>[2x]AAAAALSTLSSTESLTISSNRTLVSPGNIFELGFFRTNSRWYLGMWYKKLSGRTYVWVANRDNPLSNSIGTLKISNMNLVLLDHSNKSVWSTNLTRENVRSPVVAELLANGNFVVRDPSGFLWQSFDYPTDTLLPEMKLGYDLKTGLNRFLVSW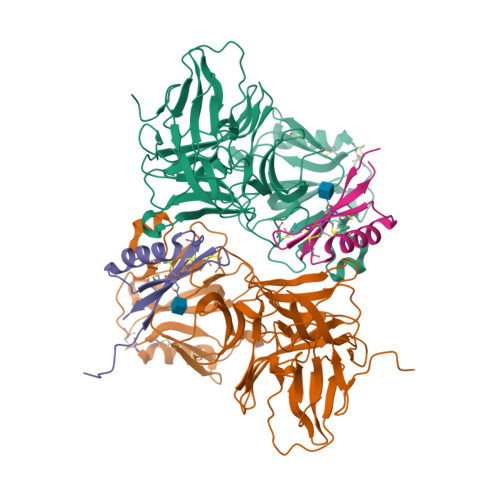RSSDDPSSGDFSYKLDIQRGLPEFYTFKDNTLVHRTGPWNGIRFSGIPEEQQLSYMVYNFTENSEEVAYTFLVTNNSIYSRLTINFSGFFERLTWTPSLVIWNPIWSSPASFQCDPYMICGPGSYCDVNTLPLCNCIQGFKPLNVQEWDMRDHTRGCIRRTRLSCRGDGFTRMKNMKLPETTMATVDRSIGVKECEKKCLSDCNCTAFANADIRDGGTGCVIWTGRLDDMRNYAVSGQDLYVRLAAADVVE;>[2x]AAANLRKTCVHRLNSGGSCGKSGQHDCEAFYTNKTNQKAFYCNCTSPFRTRYCDCAIAA>VAFGADAAKTTQEKFDALKEAGVFSGYPGTTDAKLGQDMTRAEFAKVLVKLFGLKEIHGQYSYKDKNYDAKNWAAPFIEAVTAEGLMQGKDLTKKIFDFNGKITVEEASKTLVTALKLEPVKDAQNKATDWAKGYFEAAVNAGLFSKDANPKANATRAQLVEAAFAADEMSKGSGSHHHHHH[2x]

Prokaryotic cell envelopes often include proteinaceous surface (S-) layers composed of self-assembling subunits in porous two-dimensional crystalline lattices. S-layer anchoring is best characterized for Gram-positive bacteria, where S-layer proteins non-covalently attach to the PG layer via species- and strain-specific non-classical secondary cell wall polymers (SCWPs). SpaA possesses three consecutive SLH domains near its N-terminus, followed by a large C-terminal region presumed to harbor the self-assembling domain(s). The crystal structures and binding analyses presented here of P. alvei SpaASLH, SpaASLH/G109A, and SpaASLH/G46A/G109A with synthetic SCWP fragments provide novel insights into the functional contributions of many conserved SLH domain residues, including SLH-Trp13, SLH-Gly29, and SLH-Arg43, which precisely interlock from three different SLH domains to generate two active binding sites.

To investigate the molecular details of SCWP binding by SLH domains, we synthesized the monosaccharide 4,6-Pyr-β-d-ManNAcOMe, which represents the pyruvylated moiety of P. alvei SCWP, and co-crystallized it with SpaASLH. The first co-crystal structure determined reveals ligand bound in G2 only, in a narrow pocket formed by conserved residues from all three SLH domains: Arg61 (corresponding to the conserved SLH-Arg43 of the TRAE motif) from SLH1; Met107, Gln108, Gly109 (corresponding to the conserved SLH-Gly29), Lys110, Glu127, and Lys130 from SLH2; and Trp151 (corresponding to the conserved SLH-Trp13) from SLH3. The pyruvate moiety of the ligand is bound deep in the pocket through salt bridge interactions to Arg61 and Lys130 and hydrogen bonds to Gln108 and Gly109 backbone amides, while the hydrophobic face of the ManNAc ring stacks against Trp151. To further investigate the activity of these two potential binding sites, we performed isothermal titration calorimetry (ITC) analysis of SpaASLH binding to 4,6-Pyr-β-d-ManNAcOMe in solution, which revealed 1:1 binding with an apparent dissociation constant (KD) of 29 nM. Upon binding in G2 of wt SpaASLH, the phi angle of Gly109 (SLH-Gly29) and the psi angle of Gln108 (SLH-28) each flip by ~180°. The backbone carbonyl of Gln108, which hydrogen bonds to Arg61 (the conserved SLH-Arg43) when unliganded, is resultantly replaced in space by the Gly109 backbone amide nitrogen, which forms a hydrogen bond to a pyruvyl carboxyl of ligand. Concurrently, the removal of the hydrogen bond between Gln108 and Arg61 allows Arg61 to make a bidentate interaction with a pyruvyl carboxyl and O6 of ligand. The backbone flip requires the flexibility of SLH-Gly29 in this location as the resulting phi–psi angles are disallowed for all other amino acids. Therefore, the near universal conservation of SLH-Gly29 suggests that this backbone flip is part of a conserved mechanism for SLH–SCWP binding.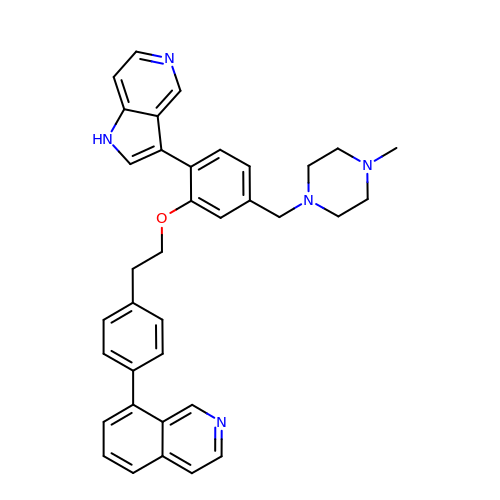8-[4-(2-{5-[(4-methylpiperazin-1-yl)methyl]-2-(1H-pyrrolo[3,2-c]pyridin-3-yl)phenoxy}ethyl)phenyl]isoquinoline | C36 H35 N5 O | KOBJJEIVOKWSMI-UHFFFAOYSA-N>[2x]MLY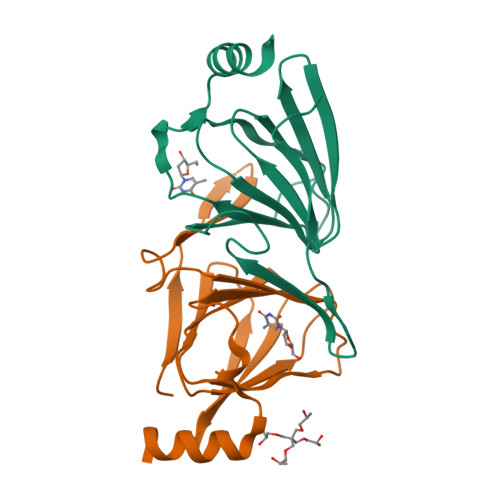NVALIKFKDIADKYGHLTPIEGKIDIPFDIKRVYYITKVDKDITRGYHSHKKLHQVLICLNGSVKIRLKIPDEEKIIELNDPSVGLYIGPLVWREMFDFTEGCVLLVLASEYYDETDYIRNYDFYIDEAKKRFLEHHHHHH METHYL-CARBAMIC ACID ETHYL ESTER 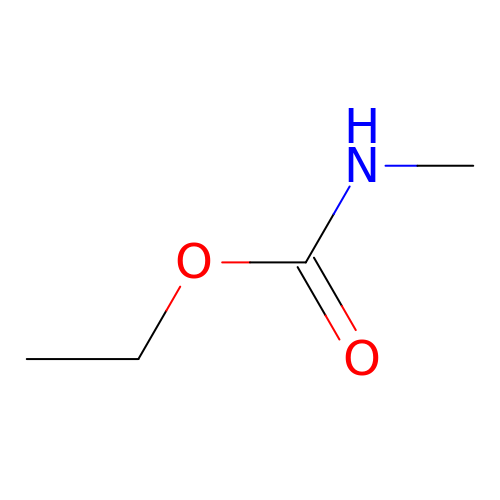| C4 H9 N O2 | SURZCVYFPAXNGN-UHFFFAOYSA-N> MKTTTPLVHVASVEKGRSYEDFQKVYNAIALKLREDDEYDNYIGYGPVLVRLAWHISGTWDKHDNTGGSYGGTYRFKKEFNDPSNAGLQNGFKFLEPIHKEFPWISSGDLFSLGGVTAVQEMQGPKIPWRCGRVDTPEDTTPDNGRLPDADKDAGYVRTFFQRLNMNDREVVALMGAHALGKTHLKNSGYEGGGANNVFTNEFYLNLLNEDWKLEKNDANNEQWDSKSGYMMLPTDYSLIQDPKYLSIV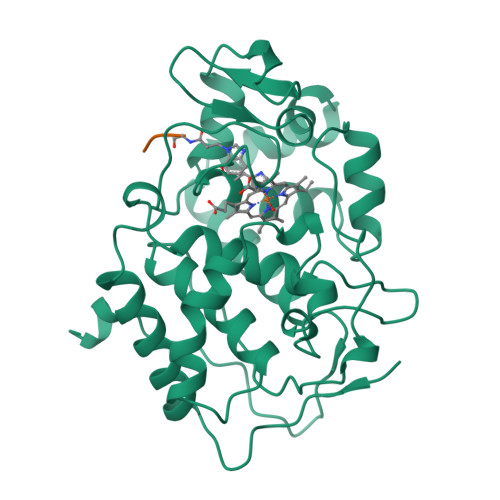KEYANDQDKFFKDFSKAFEKLLENGITFPKDAPSPFIFKTLEEQGL>GDYKEEEEIVEIDEEDAAMFEQYFKKSDDFNSLSGSYNLADKIMASIREKESQVEDMQDDEPLANEQNTSRGNISSGLKSGEGVALPEKVIKAYTTVGSILKTWTHGKLPKLFKVIPSLRNWQDVIYVTNPEEWSPHVVYEATKLFVSNLTAKESQKFINLILLERFRDNIETSEDHSLNYHIYRAVKKSLYKPSAFFKGFLFPLVETGCNVREATIAGSVLAKVSVPALHSSAALSYLLRLPFSPPTTVFIKILLDKKYALPYQTVDDCVYYFMRFRILDDGSNGED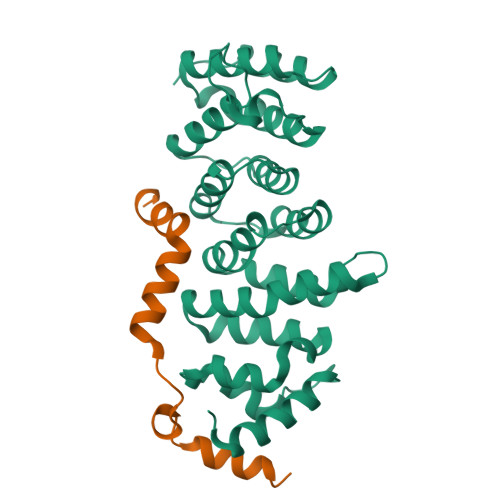ATRVLPVIWHKAFLTFAQRYKNDITQDQRDFLLETVRQRGHKDIGPEIRRELLAGASREFVDPQEANDDLMIDVN[2x];> GAMSDVSGFSMSSSAIARTETMTVLDDQYDQIINGYENYEEELEEDEEQNYQPFDMSAERSDFESMLDDFLDNYELESGGRKLAKKDKEIERLKEAADEVSKGKLSQRRNRERQEKKKLEKVTNTLSSLKF> GAMANKAPSQMERSITTIIDTFHQYSRKEGHPDTLSKKEFRQMVEAQLATFMKKEKRNEALINDIMEDLDTNQDNQLSFEECMMLMAKLIFACHEKLHENN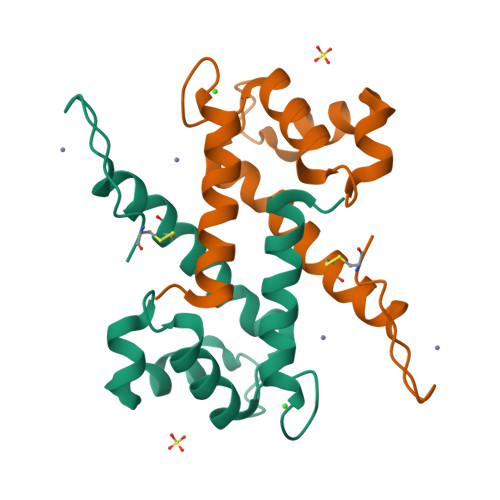PRGHGHSHGKGCGK>TDKLTSLRQYTTVVADTGDIAAMKLYQPQDATTNPSLILNAAQIPEYRKLIDDAVAWAKQQSNDRAQQIVDATDKLAVNIGLEILKLVPGRISTEVDARLSYDTEASIAKAKRLIKLYNDAGISNDRILIKLASTWQGIRAAEQLEKEGINCNLALLFSFAQARACAEAGVFLISPFVGRILDWYKANTDKKEYAPAEDPGVVSVSEIYQYYKEHGYETVVMGASFRNIGEILELAGCDRLTIAPALLKELAESEGAIERKLSYTGEVKARPARITESEFLWQHNQDPMAVDKLAEGIRKFAIDQEKLEKMIGDLL[2x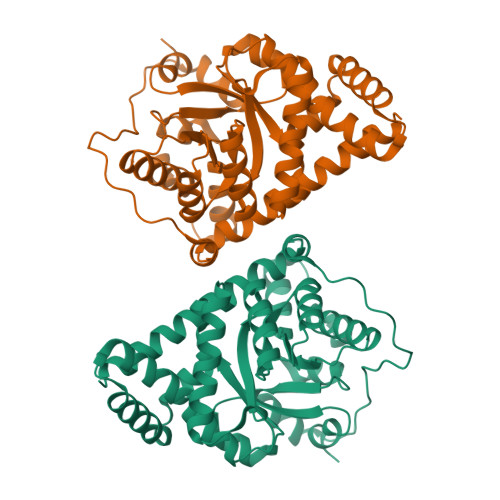]>MGRRRSHERRDLPPNLYIRNNGYYCYRDPRTGKEFGLGRDRRIAITEAIQANIELFSGHKHKPLTARINSDNSVTLHSWLDRYEKILASRGIKQKTLINYMSKIKAIRRGLPDAPLEDITTKEIAAMLNGYIDEGKAASAKLIRSTLSDAFREAIAEGHITTNHVAATRAAKSEVRRSRLTADEYLKIYQAAESSPCWLRLAMELAVVTGQRVGDLCEMKWSDIVDGYLYVEQSKTGVKIAIPTALHIDALGISMKETLDKCKEILGGETIIASTRREPLSSGTVSRYFMRARKASGLSFEGDPPTFHELRSLSARLYEKQISDKFAQHLLGHKSDTMASQFRDDRGREWDKIEIK[4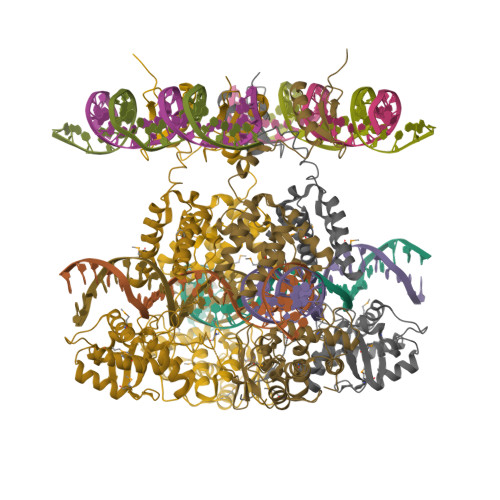x]(2R,3R,4S)-2-({[(1R)-2-HYDROXY-1-PHENYLETHYL]AMINO}METHYL)PYRROLIDINE-3,4-DIOL 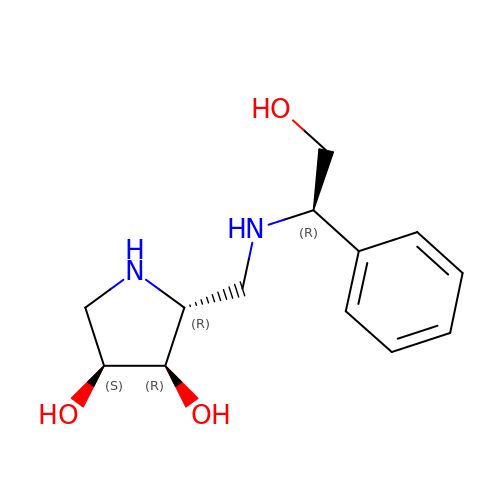| C13 H20 N2 O3 | OGMKEJTXCCFISS-MROQNXINSA-N> SFVKDFKPQALGDTNLFKPIKIGNNELLHRAVIPPLTRMRALHPGNIPNRDWAVEYYTQRAQRPGTMIITEGAFISPQAGGYDNAPGVWSEEQMVEWTKIFNAIHEKKSFVWVQLAVLGWAAFPDNLARDGLRYDSASDNVFMDAEQEAKAKKANNPQHSLTKDEIKQYIKEYVQAAKNSIAAGADGVEIHSANGYLLNQFLDPHSNTRTDEYGGSIENRARFTLEVVDALVEAIGH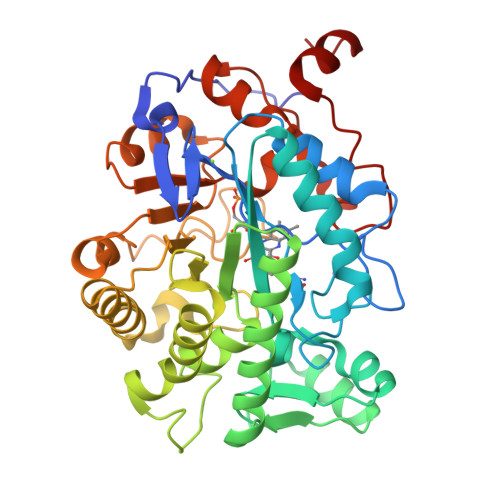EKVGLRLSPYGVFNSMSGGAETGIVAQYAYVAGELEKRAKAGKRLAFVHLVEPRVTNPFLTEGEGEYEGGSNDFVYSIWKGPVIRAGNFALHPEVVREEVKDKRTLIGYGRFFISNPDLVDRLEKGLPLNKYDRDTFYQMSAHGYIDYPTYEEALKLGWD> MKNKVQLITYADRLGDGTIKSMTDILRTRFDGVYDGVHILPFFTPFDGADAGFDPIDHTKVDERLGSWDDVAELSKTHNIMVDAIVNHMSWESKQFQDVLAKGEESEYYPMFLTMSSVFPNGATEEDLAGIYRPRPGLPFTHYKFAGKTRL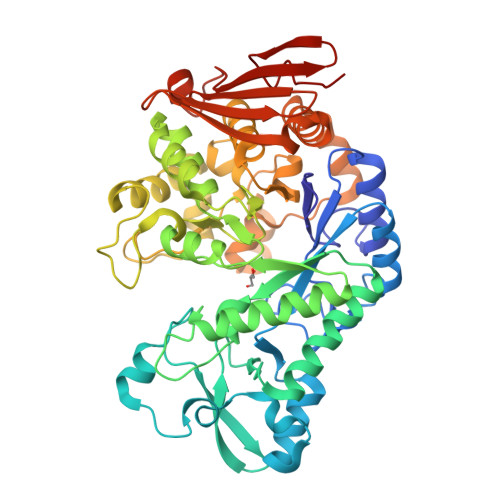VWVSFTPQQVDIDTDSDKGWEYLMSIFDQMAASHVSYIRLDAVGYGAKEAGTSCFMTPKTFKLISRLREEGVKRGLEILIEVHSYYKKQVEIASKVDRVYDFALPPLLLHALSTGHVEPVAHWTDIRPNNAVTVLDTHDGIGVIDIGSDQLDRSLKGLVPDEDVDNLVNTIHANTHGESQAATGAAASNLDLYFVNSTYYSALGCNDQHYIAARAVQFFLPGVPQVYYVGALAGKNDMELLRKTNNGRDINRHYYSTAEIDENLKRPVVKALNALAKFRNELDAFDGTFSYTTDDDTSISFTWRGETSQATLTFEPKRGLGVDNTTPVAMLEWEDSAGDHRSDDLIANPPVVA>REVLTGGHSVSAPQENRIYVMDSVFMHLTESRVHVYDYTNGKFLGMVPTAFNGHVQVSNDGKKIYTMTTYHERITRGKRSDVVEVWDADKLTFEKEISLPPKRVQGLNYDGLFRQTTDGKFIVLQNASPATSIGIVDVAKGDYVEDVTAAAGCWSVIPQPNRPRSFMTICGDGGLLTINLGEDGKVASQSRSKQMFSVKDDPIFIAPALDKDKAHFVSYYGNVYSADFSGDEVKVDGPWSLLNDEDKAKNWVPGGYNLVGLHRASGRMYVFMHPDGKEGTHKFPAAEIWVMDTKTKQRVARIPGRDALSMTIDQQRNLMLTLDGGNVNVYDISQPEPKLLRTIEGAAEASLQVQFHPVGGT[2x];>[2x]AGGGGSSSGADHISLNPDLANEDEVNSCDYWRHCAVDGFLCSCCGGTTTTCPPGSTPSPISWIGTCHNPHDGKDYLISYHDCCGKTACG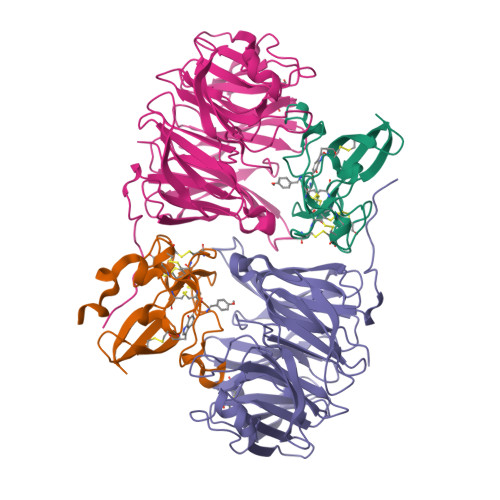RCQCNTQTRERPGYEFFLHNDVNWCMANENSTFHCTTSVLVGLAKN The Smc5/6 complex plays roles in DNA repair and in preventing the accumulation of deleterious DNA junctions. Several features make the Smc5/6 complex with its two SMC proteins (Smc5 and Smc6) and six “Non‐SMC Elements” (Nse1‐6) profoundly different from cohesin and condensin. The last two subunits, Nse5 and Nse6, form a stable heterodimer and have only very weak sequence similarity to their presumed vertebrate counterparts Slf1 and Slf2 (Raschle et al, 2015). We found that the Nse5/6 sub‐complex strongly inhibited the Smc5/6 ATPase by preventing productive ATP binding.

Limited proteolysis of purified Nse5/6 led to the design of two N‐terminally truncated Nse6 fragments (154‐C and 177‐C) which were easily co‐purified with Nse5 indicating a stable interaction with Nse5. The Nse5/Nse6(177‐C) complex yielded selenomethionine substituted protein crystals that diffracted to 3.3 Å resolution and provided experimental phase information to compute an electron density of high enough quality to build a structural model (Figs 2C and EV1). In the electron density map, residues 284–464 of Nse6 were visible, corresponding to the domain with predicted α‐helical secondary structure. It indeed folds into 11 α‐helices, arranged in an overall crescent‐shaped structure (Figs 2C and EV1A). We did not observe reliable density for Nse6 residues 177–283, indicating flexibility in this region in the crystal. For Nse5, we observed clear density for 16 α‐helices formed by residues 2–518 (Figs 2C and EV1B), with some of the helices being connected by apparently extended loops (147–197, 290–340 and 430–491), for which we only detected poor density or none at all. The Nse5/6 interaction interface covers around 1,300 Å2 in the crystal, as calculated by the PISA server. On Nse6, it mainly involves residues located in helices α3, α6, α9 and α11 together forming a concave interaction surface with a clear pattern of sequence conservation (Fig EV1A). Its pronounced hydrophobic area packs tightly against Nse5 residues forming helices α2 and α5, as well as a loop connecting helices α4 and α5. On the Nse5/6 structure, the two Nse5 lysine residues that form cross‐links to the Smc5 and Smc6 head domains are located in a loop between helices α6 and α7. Interestingly, this loop protrudes from the structure next to a highly conserved surface patch, supporting the hypothesis that this region is involved in interaction between Smc5/6 and Nse5/6 complexes.

> GPAAMSGSIPEIYLDVVTKETISDKYKDWHFISKNCHYEQLMDLEMKDTAYSFLFGSSRSQGKVPEFVHLKCPSITNLLVLFGVNQEKCNSLKINYEKKENSRYDNLCTIFPVNKMLKFLMYFYSDDDNDDVREFFLKAFICLILDRKVFNAMESDHRLCFKVLELFNEAHFINSYFEIVDKNDFFLHYRLLQIFPHLQSALLRRRFSEKQGRTETIQQNIIKEFNEFFDCKNYKNLLYFILTMYGSKFIPFGPKCQVTEYFKDCILDISNETTNDVEISILKGILNLFSKIRGXXXXXXXXXXXXXX;> MDGALINSVLYVSPRNGAHYFVELTEKHLLAFEMLNSMCLLENYDHVLLFLECQFGKSHNLAVIPFDIILVLFTLSTLSEYYKEPILRANDPYNTSRETLSRRALKLLQKYLAILKEFDSEQYNLYDLELLRCQFFLAIDTLTPKKQKWGFDRFRRTKSESGVTYRQNASVDPELDQAKTFKNPYRSYISCLEQRNTILGNRLLNLKLNEPGEFINMILWTLSNSLQESTPLFLSSHEIWMPLLEILIDLFSCRQDYFIQHEVAQNVSKSLFVQRLSESPLAVFFESLNTRNFANRFSEYVFLNCDYKLPSDNYATPVHPVYNGENTIVDTYIPTIKCSPLYKSQKSLALRRKLIGSCFKLLLRVPDGHRLITPRIVADDVIQGISRTLASFNDILQFKKFFMTENLSQESYFIPLLAEGTLSEILKDTQECVVILTLVENLSDGVSFCNEVIGLVKSKCFAFTEQCSQASYEEAVLNIEKCDVCLLVLLRYLLHLIGTEAILDAKEQLEMLHAIEKNDSGRRQWAKALNLGNDPPLLYPIVSQMFGVHDKSVIIEXXXXXXXXXXXXXXXXXXXXXXXXXXXXXXXXXXXXXXXXXXXXXXXXXXX>AMSKIICLTAGHSNTDPGAVNGSDREADLAQDMRNIVASILRNDYGLTVKTDGTGKGNMPLRDAVKLIRGSDVAIEFHTNAAANKTATGIEALSTPKNKRWCQVLGKAVAKKTGWKLRGEDGFKPDNAGQHSRLAYAQAGGIVFEPFFISNDTDLALFKTTKWGICRAIA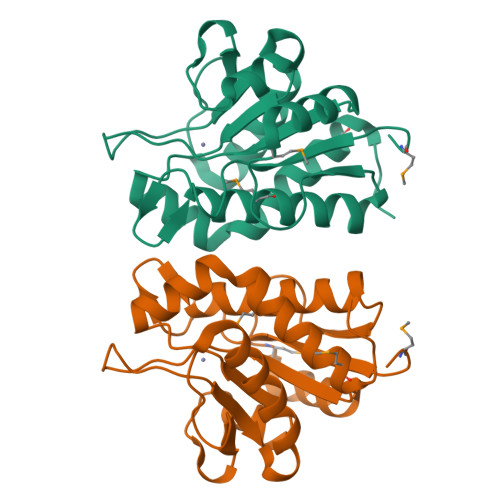DAIAMELGAAKV[4x]> MALKKNTHNKSTKRVTKHPSLKTLTHKQIHTTIFVKSTTPYVSALKRINKFLDSVHKQGSSYVAVLGMGKAVEKTLALG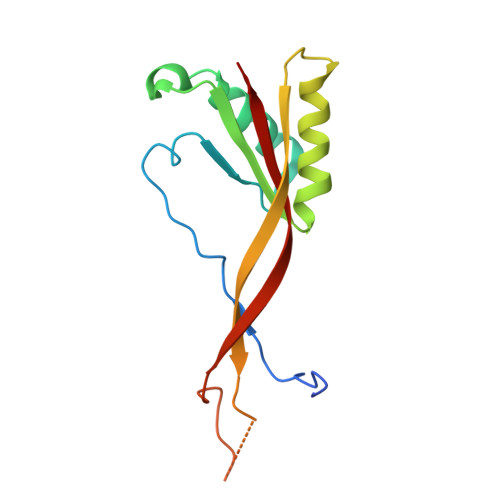CHFQDQKNKKIEVYTKTIEVLDEVITEGQADIDMESDVEDDDKETQLKKRAVSGVELRIYV>GPSGMILKRAYDVTPQKISTDKVRGVRKRVLIGLKDAPNFVMRLFTVEPGGLIDRHSHPWEHEIFVLKGKLTVLKE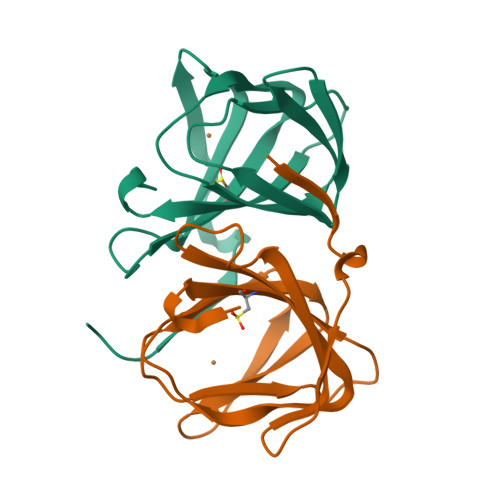QGEETVEEGFYIFVEPNEIHGFRNDTDSEVEFLCLIPKEGGE[2x]> TLSILVAHDLQRVIGFENQLPWHLPNDLKHVKKLSTGHTLVMGRKTFESIGKPLPNRRNVVLT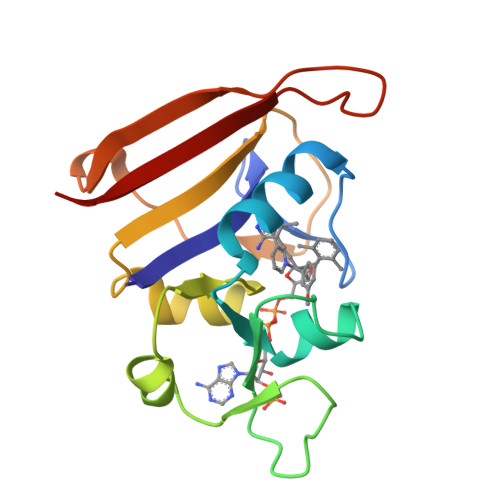SDTSFNVEGVDVIHSIEDIYQLPGHVFIFGGQTLYEEMIDKVDDMYITVIEGKFRGDTFFPPYTFEDWEVASSVEGKLDEKNTIPHTFLHLIRK>GAMEMLPNQTIYINNLNEKIKKEELKKSLYAIFSQFGQILDIVALKTLKMRGQAFVIFKEIGSASNAL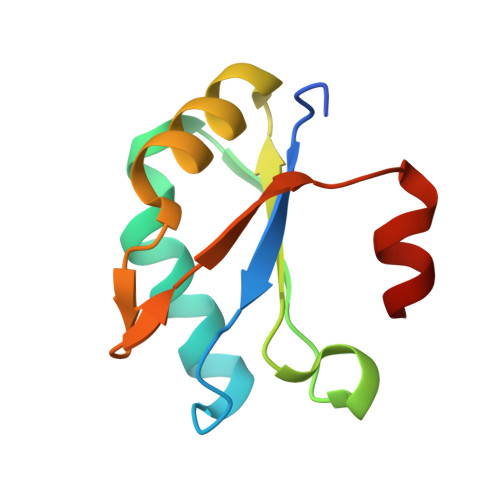RTMQGFPFYDKPMQIAYSKSDSDIVAKIKG[6x]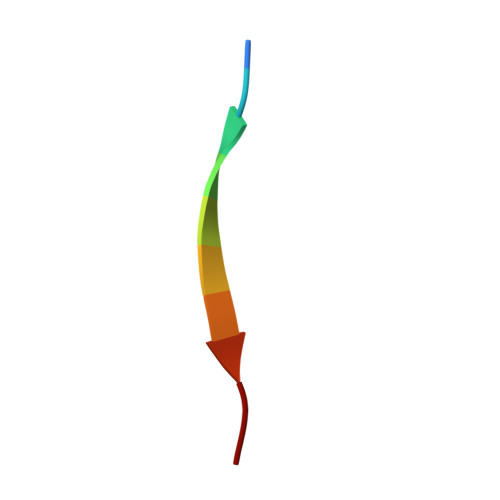> QPISVTMVTP> GMLTGCSRR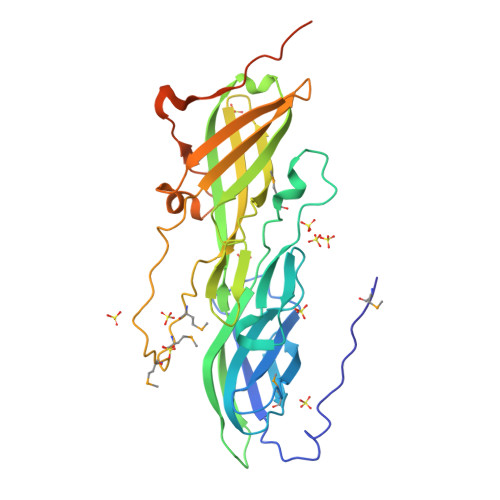DILDDYPVSGVDIKLDWDGVTDQLPEGVRVIFYPKNGDGRKVDKYLSVRGGEMKVPPGRYSVVVYNYNTESIRIRGEESYETIEAYTGNCNGLGIEGTEKMVWSPDSLYVLNIDELKIEKSEEVLRLDWKLESVVKKYSFAVEAKGLEYVATVVGSIDGLSDCYCIGKGRGVCSSQPIYFEVKKGDNKVTAFFTAFKQVKEMTMPTRMSTSERETSSEKGAIILILKFIKTDNTVQEATIDVTEIIGTLENAGTGEDGKPTPPPEIELPPDDKIEVDKPETPPNPDGGGGMGGNVDGWGPEDNVELPVN> AYVINEA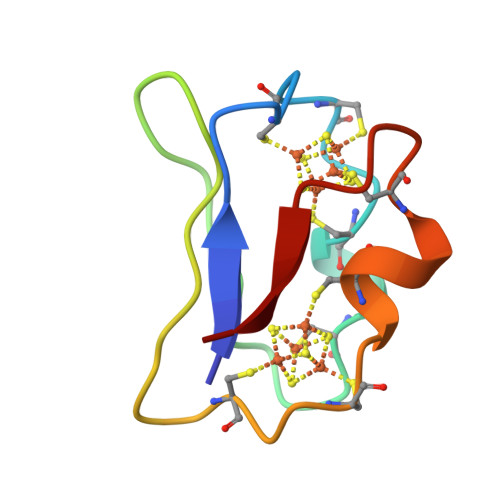CISCGACEPECPVNAISSGDDRYVIDADTCIDCGACAGVCPVDAPVQA>ANEGDVYKCELCGQVVKVLEEGGG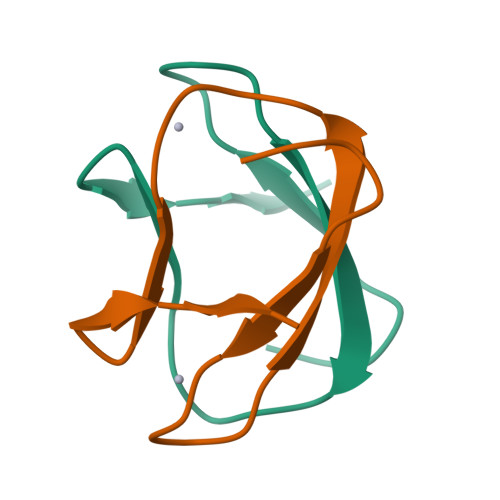TLVCCGEDMVKQ[2x]> MESKNKTAATQQSEPNVIAAHKGVNQAPVPLKMERVGPHDVHIEMTAQITDIEIDKGKIYKAWTFNGQAPGPLVVVNEGDTIHFTLKNMDPVVPHSMNFHAVHASPSKDFIDVMPNKSGTFTYPANKPGVFMYHAATKPVLQHIANGMHGVIIVKPKNGYPTDKEVDREYVLIQNEWYKYNDMNDFQNGVPSYVVFSSKALKPGDPNTNGDTFTLKEKPLLAKVGEKIRLYINNVGPNEVSSFHVVGTVFDDVYLDGNPNNHLQGMQTVMLPASGGAVVEFTVTRPGTYPIVTHQFNHAQKGAVAMLKVTETGEDDGTETSGH

Copper-containing nitrite reductases (CuNIRs) catalyze transformation of nitrite to nitric oxide, which has impacts on geochemical, agricultural, and medical health fields. CuNIRs typically have an ∼110 kDa homotrimeric structure, like a Reuleaux triangle. Each protomer contains one type 1 copper (T1Cu) and one type 2 copper (T2Cu) site. The Cys residue forms a peptide-bond bridge (Cys-His bridge) together with one of the His ligands at the T2Cu site to transfer the electron to the catalytic T2Cu site, which is coordinated by three His residues and an axial water molecule.

Since the GK-like conformer complicates the interpretation of the T2Cu site structure, we constructed D98N/G136A and D98N/C135A/G136A mutants. The structures of D98N/G136A without NO2- and D98N/C135A/G136A in complex with NO2- were determined at 0.96 and 0.99 Å resolution, respectively. As was expected, Asn98 does not exhibit the GK-like conformation in either of the G136A-containing mutants. However, NO2- again shows several coordination manners in the D98N/C135A/G136A structure, indicating that the GK-like conformation observed in the D98N/C135A mutant is not responsible for the multiple conformers of NO2-. The first conformation of NO2- in the D98N/C135A/G136A structure is the κ1-O mode that is observed in the native T2Cu site. In this state, the distance between NO2- and the amide N atom of Asn98 is 3.2 Å, which is identical to that between AspCAT and NO2- observed in the neutron structure. The second binding mode is the complete κ2-O,O coordination in the vertical mode. This state shows a shorter distance to the side chain amide N atom of Asn98 (2.9 Å) than that in the neutron structure. Because the complete κ2-O,O bidentate mode is typical of the D98N mutants, the hydrogen bond with AspCAT is necessary for stabilization of the κ2-O,O mode. The third binding mode is the κ1-N mode that is also observed in the C135A/D98N structure.> ETLVRPKPLLLKLLKSVGAQKDTYTMKEVLFYLGQYIMTK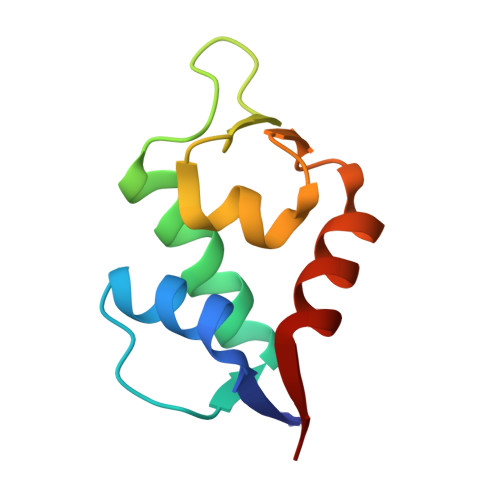RLYDEKQQHIVYCSNDLLGDLFGAPSFSVKEHRKIYTMIYRNLVVV>GAMEDPVEYPADYFRKSKEIPLYINTTKSLSDLRGYVYQGLKSGNVSIIHVNSYLYGALKDIRGKLDKDWSSFGINIGKAGDTIGIFDLVSLKALDGVLPDGVSDASRTSADDKWLPLYLLGLYRVGRTQMPEYRKKLMDGLTNQCKMINEQFEPLVPEGRDIFDVWGNDSNYTKIVAAVDMFFHMFKKHECASFRYGTIVSRFKDCAALATFGHLCKITGMSTEDVTTWILNREVADEMVQMMLPGQEIDKADSYMPYLIDFGLSSKSPYSSVKNPAFHFWGQLTALLLRSTRARNARQPDDIEYTSLTTAGLLYAYAVGSSADLAQQFCVGDNKYT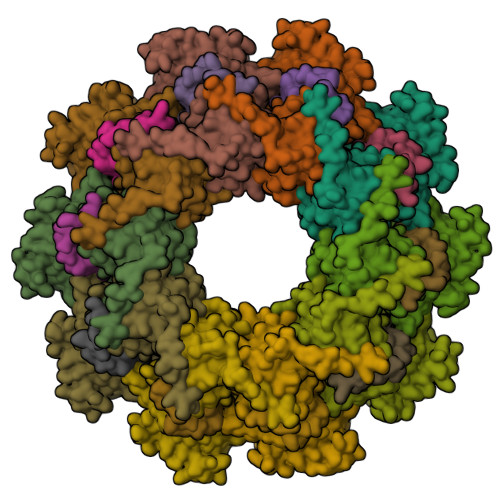PDDSTGGLTTNAPPQGRDVVEWLGWFEDQNRKPTPDMMQYAKRAVMSLQGLREKTIGKYAKSEFDK[5x];>[5x]MDNLTKVREYLKSYSRLDQAVGEIDEIEAQRAEKSNYELFQEDGVEEHTKPSYFQAADDSLEHHHHHH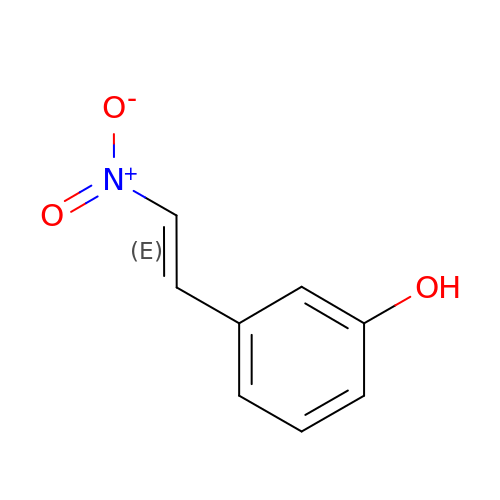3-[(E)-2-nitroethenyl]phenol | C8 H7 N O3 | DHTXBJQMDPODIB-SNAWJCMRSA-N> MSHHHHHHGSSRQANRGTESKKMSSELFTLTYGALVTQLCKDYENDEDVNKQLDKMGFNIGVRLIEDFLARSNVGRCHDFRETADVIAKVAFKMYLGITPSITNWS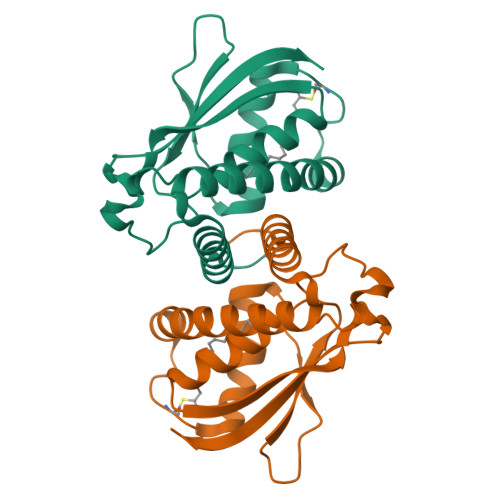PAGDEFSLILENNPLVDFVELPDNHSSLIYSNLLCGVLRGALEMVQMAVEAKFVQDTLKGDGVTEIRMRFIRRIEDNLPAGEEAAAWSHPQFEK> MTTVTSYPGVYIEELNSLALSVSNSATAVPVFAVDEQNQYISEDNAIRINSWMDYLNLIGNFNNEDKLDVSVRAYFANGGGYCYLVKTTSLEKIIPTLDDVTLLVAAGEDIKTTVDVLCQPGKGLFAVFDGPETELTINGAEEAKQAYTATPFAAVYYPWLKADWANIDIPPSAVMAGVYASVDLSRGVWKAPANVALKGGLEPKFLVTDELQGEYNTGRAINMIRNFSNTGTTVWGARTLEDKDNWRYVPVRRLFNSVERDIKRAMSFAMFEPNNQPTWERVRAAISNYLYSLWQQGGLAGSKEEDAYFVQIGKGITMTQEQIDAGQMIVKVGLAAVRPAEFIILQFTQ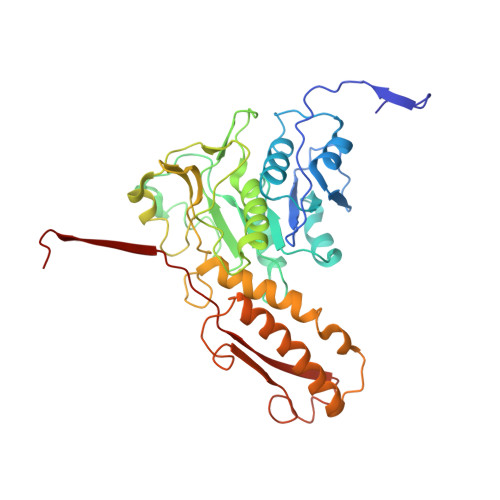DVEQR>MGHHHHHHGAASIGYKRESGARLRTTADMFKDHLNLKEYCPGDGTNQTTAFNAAIARAVSEGISRIIVPAGHYLVTDLSVTANGLVFEGQGESSRIQVASNNSRCFSLSGDRLTFRGLKFIGDGTASASANGIGILAGDATDLLVEDVWFDSFGFGGVNA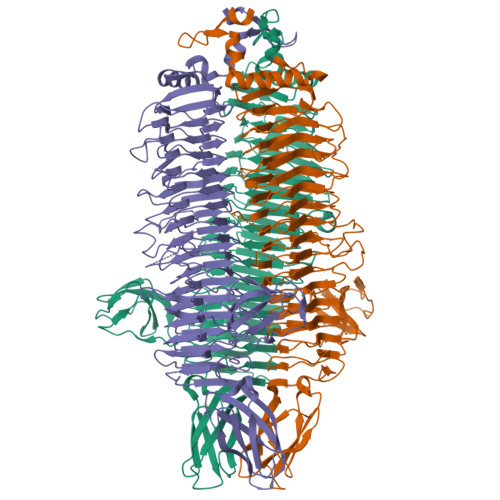GFTTLARGPKFIRTRHRNTGTGGAEIYLRGLYEGADVIDIDAATSNADWAVFAFDEGYAGQRDLEVTRGDFSGYKRYSIGVSDENPSGEDRGFGVKINGGHHKNAGLGAVKVKNYRGVLIQGVTTDNCGIVPIAGISNTGESGTFYINSAGLVDIGGCKLRDNGMDGITVIQGAPYPTTNADGTARNQYIVHDNQIDGCGTASYAGTGTGFRIKSGVHQAFLTNNSARGCTRFVAELGNDPSNISETITVIGNDFSQNLSATNGIYARYINRLKMDMNQIENTGAQVVYGLDIDTVYSGPGDRFGNNTVADFHVRFDSCRDLTLLGDYSSTDYTQWVTATAVPVGAKRWNGANAYVAEAAGTTGATAPTHTSGTVSDGGVNWRYIGKRRIAAAAVALRGTAAALVRMGGTTRTNSTSTAHGIDFSPSPTRWEWSDIDAGTATLAAGTVTVNITDNRRQVDGNYRVLVTGTVNETFYVSARAASNFTITSSNAASTATVMWKIFR[3x]>MNAKTKFDLYQHVTDRIIASIEAGTPAWRKPWTGEAATMQMPLRSNGEAYRGINVVMLWLTAAEKGYRSAYWFTYRQAKELGGQVRKGEKGSTVVKFGTIEREDEQTGEEKKIPYLKGYTVFNADQIDGLPEQYHAAPAEAARDLGTAADPELDAFFAATGADIRTSS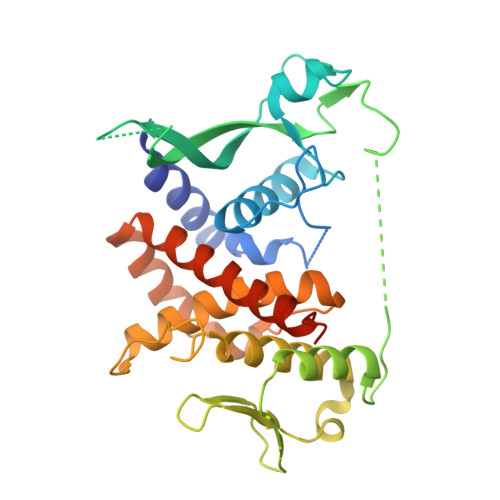EPRAYYNPTGDYIHMPPIATFHSAAGYYATLAHEATHWTGHKSRLDRFSRFSDRKSYAFEELIAEIGNCMLCASLGLIPDFDQSAAYVQSWLRALKDDKRLIFKAATEAQKAADLLQENAANFQRKEAALEHHHHHH[8x]>SMGKVNVAKLRYMSRDDFRVLTAVEMGMKNHEIVPGSLIASIASLKHGGCNKVLRELVKHKLIAWERTKTVQGYRLTNAGYDYLALKTLSSRQVVESVGNQMGVGKESDIYIVANEEGQQFALKLHRLGRTSFRNLKNKRDYHKYRHNVSWLYLSRLSAMKEFAYMKALYERKFPVPKPIDYNRHAVVMELINGYPLCQIHHVEDPASVYDEAMELIVKLANHGLIHGDFNEFNLILDESDHITMIDFPQMVSTSHPNAEWYFDRDVKCIKDF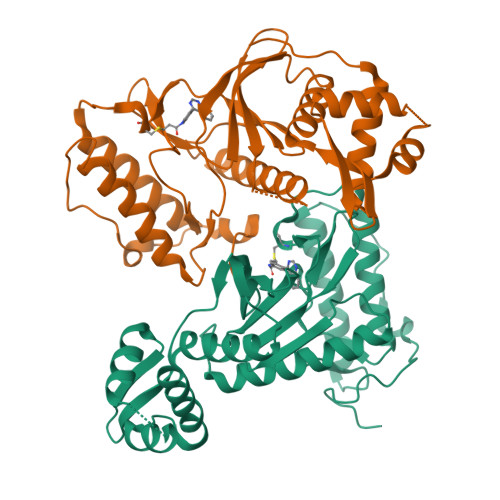FMKRFSYESELFPTFKDIRREDTLDVEVSASGYTKEMQADDELLHPLGPDDKNIETK[2x]>MHHHHHHSAGENLYFQGKEWQENKSWNAHFTEHKSQGVVVLWNENKQQGFTNNLKRANQA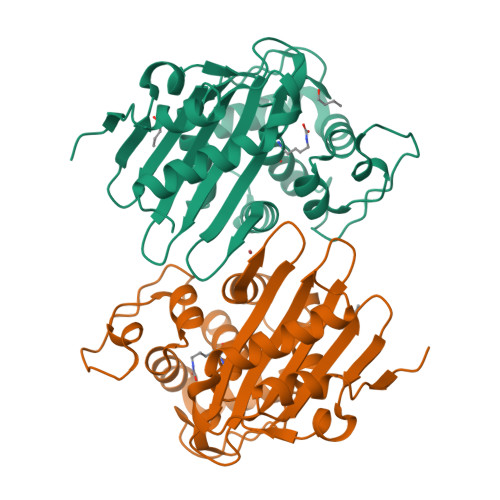FLPASTFKIPNSLIALDLGVVKDEHQVFKWDGQTRDIATWNRDHNLITAMKYSVVPVYQEFARQIGEARMSKMLHAFDYGNEDISGNVDSFWLDGGIRISATEQISFLRKLYHNKLHVSERSQRIVKQAMLTEANGDYIIRAKTGYSTRIEPKIGWWVGWVELDDNVWFFAMNMDMPTSDGLGLAQAITKEVLKQEKIIP[4x]>GPGSGQEGLDFPEYDGVDRVINVNAKNYKNVFKKYEVLALLYHEPPEDDKASQRQFEMEELILELAAQVLEDKGVGFGLVDSEKDAAVAKKLGLTEVDSMYVFKGDEVIEYDGEFSADTIVEFLLDVLEDPVELIEGERELQAFENIEDEIKLIGYFKSKDSEHYKAFEDAAEEFHPYIPFFATFDSKVAKKLTLKLNEIDFYEAFMEEPVTIPDKPNEEEEIVNFVEEHRRSTLRKLKPESMYETWEDDMDGIHIVAFAEEADPDGFEFLETLKAVAQDNTENPDLSIIWIDPDDFPLLVPYWEKTFDIDLSAPQIGVVNVTDADSVWMEMDDEEDLPSAEELEDW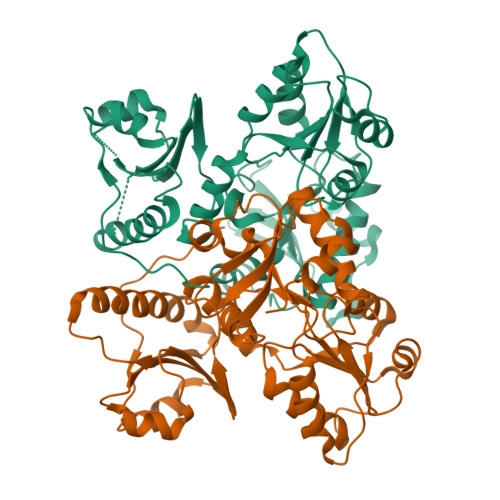LEDVLEGEINTEDDDDDDDD[2x]> MNMSQSQKIVLQPRSIVVPGELLAEGEFQIPWSPYILKINSKYYSTVVGLFDVKDTQFEVIPLEGSFYYPKINDIVIGLVEDVEIYGWVVDIKAPYKAYLPASNLLGRSINVGEDLRRYLDVGDYVIARIENFDRSIDPVLSVKGKDLGRVSNGIVIDIMPVKVPRVIGKNKSMYETLTSKSGCSIFVANNGRIWATCPS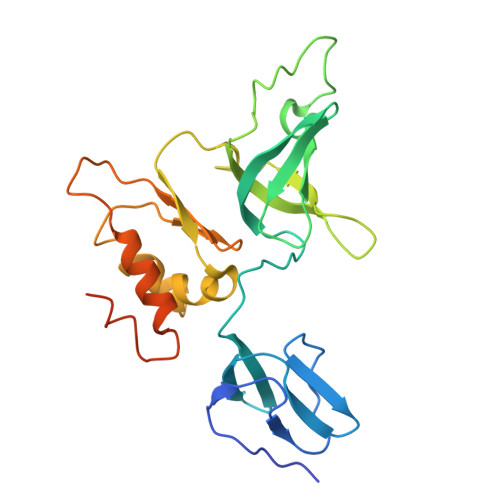RFSEEILIEAIRKIENESHIKGLTDRIKQFIEEKLGERNASSGETKTNS> GIEDLISEVAQGALTLSLPKQQDSLPDTKASGPAHSKEVPALTAVETGATNPLAPSDTVQTRHVVQRRSRSESTIESFFARGACVAIIEVDNEQPTTRAQKLFAMWRITYKDTVQLRRKLELFTYSRFDMELTFVVTANFTNANNGHALNQVYQIMYIPPGAPTPKSWDDYTWQTSSNPSIFYTYGAAPARISVPYVGLANAYSHFYDGFAKVPLKTDANDQIGDSLYSAMTVDDFGVLAVRVVNDHNPTKVTSKVRIYMKPKHVRVWCPRPPRAVPYY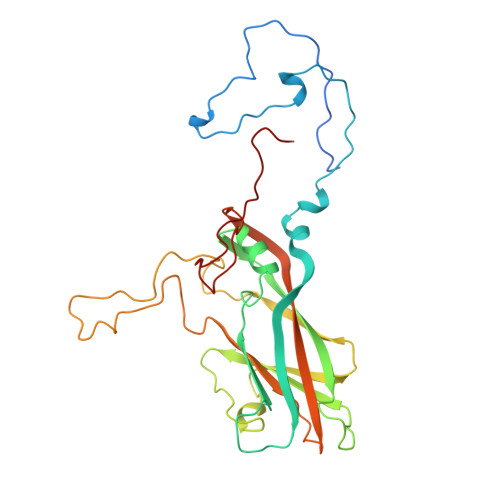GPGVDYRNNLDPLSEKGLTTY> MSQSVSERTRIKSDRYESGVIPYAKMGYWDAAYSVKDTDILALFRITPQPGVDPVEAAAAVAGESSTATWTVVWTDLLTACERYRAKAYRVDPVPNSTDVYFAFIAYECDLFEEASLSNLTASIIGNVFGFKAISALRLEDMRIPHSYLKTFQGPATGIIVERERLNKYGTPLLGATVKPKLGLSGKNYGRVVYEGLKGGLDFLKDDENINSQPFMRWRERFLNCLEGINRAAAATGEVKGSYLNITAATMEEVYKRAEYAKAIGSVVVMIDLVMGYTAIQSIAYWARENDMLLHLHRAGNSTYARQKNH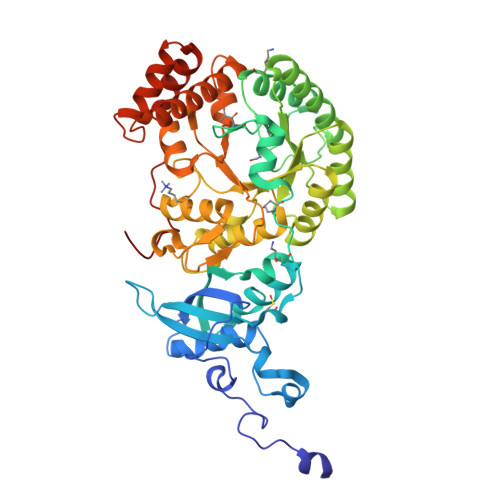GINFRVICKWMRMSGVDHIHAGTVVGKLEGDPLMIKGFYDILRLTELEVNLPFGIFFEMDWASLRRCMPVASGGIHCGQMHQLIHYLGDDVVLQFGGGTIGHPDGIQAGATANRVALEAMVLARNEGADYFNNQVGPQILRDAAKTCGPLQTALDLWKDISFNYTSTDTADFAETATANR>[2x]AFELPPLPYAHDALQPHISKETLEYHHDKHHNTYVVNLNNLVPGTPEFEGKTLEEIVKSSSGGIFNNAAQVWNHTFYWNCLSPDAGGQPTGALA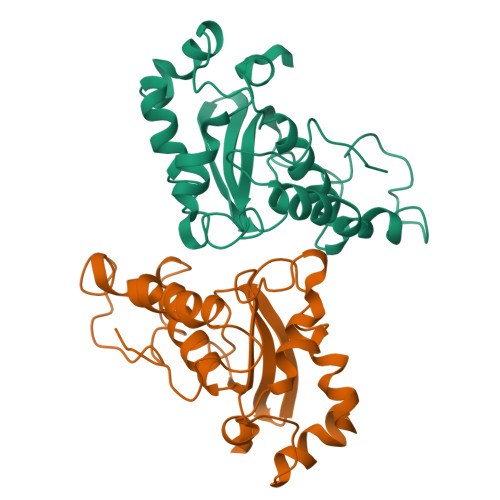DAINAAFGSFDKFKEEFTKTSVGTFGSGWAWLVKADGSLALCSTIGAGAPLTSGDTPLLTCDVWEHAYYIDYRNLRPKYVEAFWNLVNWAFVAEEGKTFKA> QDSTSDLIPAPPLSKVPLQQNFQDNQFHGKWYVVGLAGNGNLREDKDPLKMYATIYELKEDKSYNVTDVLF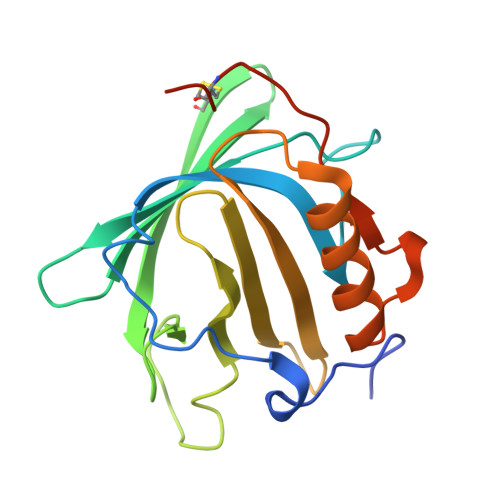IDKKCHYLINTFVPGSQPGEFTLGSIKSTLGSTSRLVRVVSTNYNQHAMVFFKWVHQNREWFYITLYGRTKELTSELKENFIRFSKSLGLPENHIVFPVPIDQCIDGSAHHHHHH>MDAMKYNDLRDFLTLLEQQGELKRITLPVDPHLEITEIADRTLRAGGPALLFENPKGYSMPVLCNLFGTPKRVAMGMGQEDVSALREVGKLLAFLKEPEPPKGFRDLFDKLPQFKQVLNMPTKRLRGAPCQQKIVSGDDVDLNRIPIMTCWPEDAAPLITWGLTVTRGPHKERQNLGIYRQQLIGKNKLIMRWLSHRGGALDYQEWCAAHPGERFPVSVALGADPATILGAVTPVPDTLSEYAFAGLLRGTKTEVVKCISNDLEVPASAEIVLEGYIEQGETAPEGPYGDHTGYYNEVDSFPVFTVTHITQREDAIYHSTYTGRPPDEPAVLGVALNEVFVPILQKQFPEIVDFYLPPEGCSYRLAVVTIKKQYAGHAKRVMMGVWSFLRQFMYTKFVIVCDDD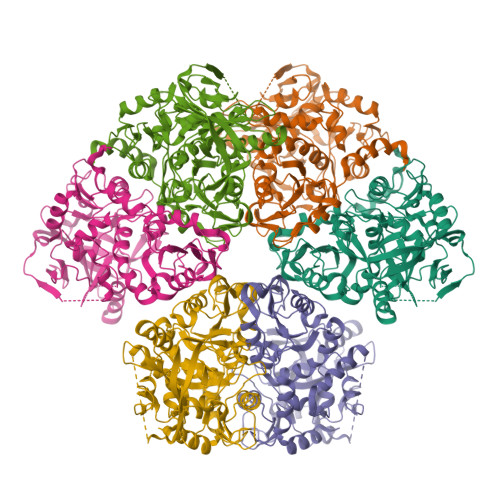VNARDWNDVIWAITTRMDPARDTVLVENTPIDYLDFASPVSGLGSKMGLDATNKWPGETQREWGRPIKKDPDVVAHIDAIWDELAIFNNGKSALEHHHHHH[3x]> GAMDPMKAKRVQAKIEIEFPSEDVAKVVYEAVLYEHLSVPYRRS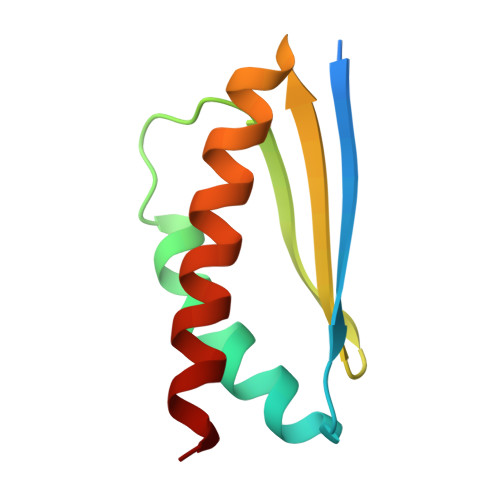EIDFKLEGKKIILDIKATDSSALRGTVNSYLRWIKAAIDVIEV>[2x]MGHHHHHHHHLVPRGSMFADLDYDIEEDKLGIPTVPGKVTLQKDAQNLIGISIGGGAQYCPCLYIVQVFDNTPAALDGTVAAGDEITGVNGRSIKGKTKVEVAKMIQEVKGEVTIHYNKLQQSAV

The C-terminus of the GluA2 subunit binds to the PDZ domain of the scaffolding PICK1 protein, an interaction that is required for AMPA receptor internalization and long term depression. Aβ produces synaptic depression by enhancing the internalization of AMPA receptors through a GluA2-dependent mechanism resulting in a reduction in the number of dendritic spines. Multiple compounds from this series were found to show a similar increase in surface GluA2 levels. These findings demonstrate that PICK1 normally functions to transport GluA2-containing AMPA receptors intracellularly, and when PICK1 is absent, the intracellular GluA2-containing receptors are released to the neuronal surface. In this study, we report the strategic use of a high throughput screen (HTS) followed by structure based drug design in combination with an array of biochemical and cellular assays in the identification of a novel, selective, and potent series of PICK1-GluA2 PDZ inhibitors.

Our next strategy was to utilize a structure-based drug design approach and visualize how the compound was interacting with the PICK1 PDZ domain by crystal structure determination of compound 1o with the PDZ domain of PICK1. We crystallized the complex using a method of protein oxidation and carboxypeptidase treatment of the “tail-biting” dimer in the presence of 1o in a similar way as described. The structure was solved using molecular replacement under standard procedures and the resulting structure was refined to an R factor of 15.5% and an Rfree of 17.7% to 1.69 Å resolution with good geometry. The overall structure of the PICK1 PDZ with compound 1o can be described as a dimer of oxidized PICK1 with two inhibitors bound in two PICK1 molecules. Similar to a 3-pronged anchor, the three hydrophobic regions of the compound (R3, R2, and R1) sit in the three peptide binding sites (S0, S−2, and S−1), respectively, leaving peptide pocket S−3 unoccupied. There is a space between the sidechains of Leu32, Asp28, and Thr56 which forms a small subpocket that is partially occupied by the CF3 group. Additionally, there are van der Waals interactions between the R2 bromophenyl group and the side chain of Lys83 and Ala87 in the S−2 pocket. Lastly, R3 of the compound nicely mimics the c-terminal amino acid of the peptide ligand and forms a hydrogen bond network with the backbone of PICK1 (Ile33, Gly34, Ile35) while the cyclopropyl alanine sidechain of R3 nicely fills the back hydrophobic pocket of S0. Compound 1o demonstrated selectivity for PICK1 over PSD95, GRIP (data not shown), and Shank PDZ domains. The compound selectivity can be attributed in part to the small size of the sidechain of Ala87, located between the S0 and S−2 pockets, which is unique to PICK1. Importantly, the selectivity may also result from interactions with the aromatic residue Phe53 (PICK1 numbering) near the S−1 pocket as only PICK1 has an aromatic residue in this position.(3aR,5S,6S,7R,7aR)-5-(difluoromethyl)-2-(ethylamino)-5,6,7,7a-tetrahydro-3aH-pyrano[3,2-d][1,3]thiazole-6,7-diol | C9 H14 F2 N2 O3 S | 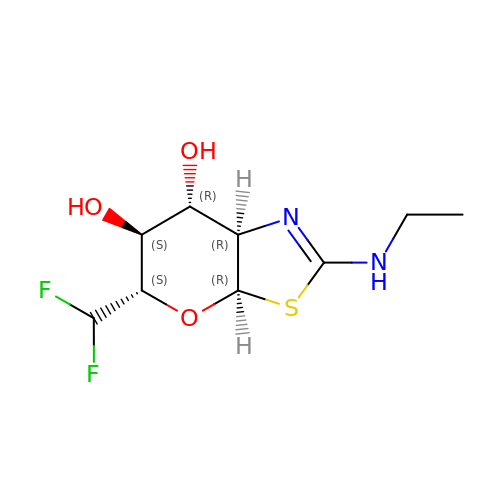UDQTXCHQKHIQMH-KYGLGHNPSA-N> GGNRTF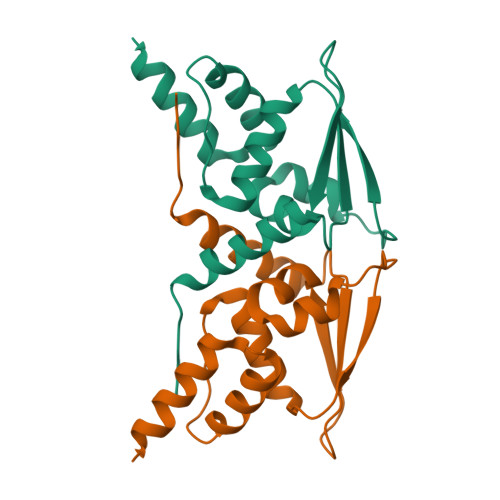SYTLEDHTKQAFGIMNELRLSQQLCDVTLQVKYQDAPAAQFMAHKAVLASSSPVFKAMFTNGLREQGMEVVSIEGIHPKVMERLIEFAYTASISMGEKCVLHVMNGAVMYQIDSVVRACADFLVQQLD>GSGGRATMEPSALRKAGSEQEEGFEGLPRRVTDLGMVSNLRRSNSSLFKSWRLQCPFGNNDKQESLSSWIPENIKKKECVYFVESSKLSDAGKVVCQCGYTHEQHLEEATKPHTFQGTQWDPKKHVQEMPTDAFGDIVFTGLSQKVKKYVRVSQDTPSSVIYHLMTQHWGLDVPNLLISVTGGAKNFNMKPRLKSIFRRGLVKVAQTTGAWIITGGSHTGVMKQVGEAVRDFSLSSSYKEGELITIGVATWGTVHRREGLIHPTGSFPAEYILDEDGQGNLTCLDSNHSHFILVDDGTHGQYGVEIPLRTRLEKFISEQTKERGGVAIKIPIVCVVLEGGPGTLHTIDNATTNGTPCVVVEGSGRVADVIAQVANLPVSDITISLIQQKLSVFFQEMFETFTESRIVEWTKKIQDIVRRRQLLTVFREGKDGQQDVDVAILQALLKASRSQDHFGHENWDHQLKLAVAWNRVDIARSEIFMDEWQWKPSDLHPTMTAALISNKPEFVKLFLENGVQLKEFVTWDTLLYLYENLDPSCLFHSKLQKVLVEDPERPACAPAAPRLQMHHVAQVLRELLGDFTQPLYPRPRHNDRLRLLLPVPHVKLNVQGVSLRSLYKRSSGHVTFTMDPIRDLLIWAIVQNRRELAGIIWAQSQDCIAAALACSKILKELSKEEEDTDSSEEMLALAEEYEHRAIGVFTECYRKDEERAQKLLTRVSEAWGKTTCLQLALEAKDMKFVSHGGIQAFLTKVWWGQLSVDNGLWRVTLCMLAFPLLLTGLISFREKRLQDVGTPAARARAFFTAPVVVFHLNILSYFAFLCLFAYVLMVDFQPVPSWCECAIYLWLFSLVCEEMRQLFYDPDECGLMKKAALYFSDFWNKLDVGAILLFVAGLTCRLIPATLYPGRVILSLDFILFCLRLMHIFTISKTLGPKIIIVKRMMKDVFFFLFLLAVWVVSFGVAKQAILIHNERRVDWLFRGAVYHSYLTIFGQIPGYIDGVNFNPEHCSPNGTDPYKPKCPESDATQQRPAFPEWLTVLLLCLYLLFTNILLLNLLIAMFNYTFQQVQEHTDQIWKFQRHDLIEEYHGRPAAPPPFILLSHLQLFIKRVVLKTPAKRHKQLKNKLEKNEEAALLSWEIYLKENYLQNRQFQQKQRPEQKIEDISNKVDAMVDLLDLDPLKRSGSMEQRLASLEEQVAQTAQALHWIVRTLRASGFSSEADVPTLASQKAAEEPDAEPGGRKKTEEPGDSYHVNARHLLYPNCPVTRFPVPNEKVPWETEFLIYDPPFYTAERKDAAAMDPMGDTLEPLSTIQYNVVDGLRDRRSFHGPYTVQAGLPLNPMGRTGLRGRGSLSCFGPNHTLYPMVTRWRRNEDGAICRKSIKKMLEVLVVKLPLSEHWALPGGSREPGEMLPRKLKRILRQEHWPSFENLLKCGMEVYKGYMDDPRNTDNAWIETVAVSV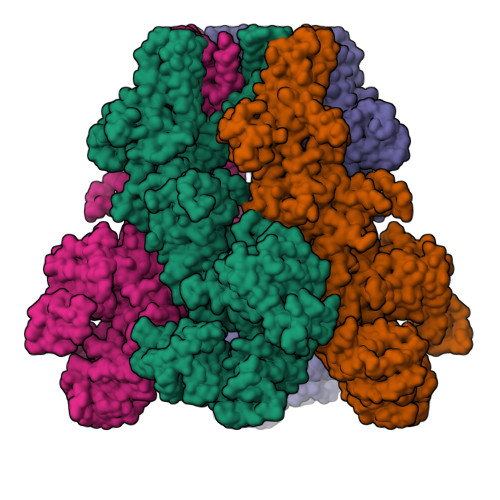HFQDQNDVELNRLNSNLHACDSGASIRWQVVDRRIPLYANHKTLLQKAAAEFGAHYFE[4x]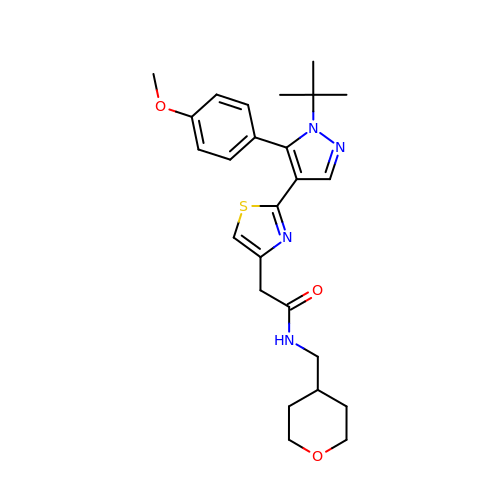2-[2-[1-~{tert}-butyl-5-(4-methoxyphenyl)pyrazol-4-yl]-1,3-thiazol-4-yl]-~{N}-(oxan-4-ylmethyl)ethanamide | C25 H32 N4 O3 S | SRKLUIJNVCRLFZ-UHFFFAOYSA-N> MGHNNTKGNRKFIKGRYTANAAKGERLVSSEFLLTFAGHEDISVLVRTS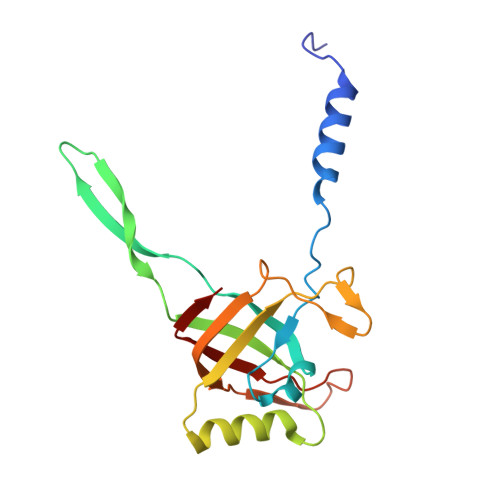QIPEMTREDVEDYGPNGVKFNQHGPIRNSGEIQVQCVETIEGDILQFIKDRIAAKDYVDITMAATPESKSSGVNAVTKAATTIEMLDCKIYSDAIDFSTEDVTAAVRPSLRIVYNWIEWD6-amino-4-[2-(benzylamino)ethyl]-2-(methylamino)-1,7-dihydro-8H-imidazo[4,5-g]quinazolin-8-one | C19 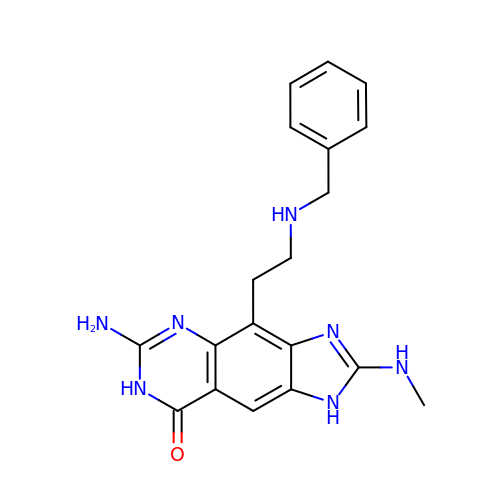H21 N7 O | OCMHTFVKOKFMET-UHFFFAOYSA-N Maintaining the optimal nucleotide balance required for normal cell proliferation is controlled by 5′-nucleotidases amongst other processes. These enzymes catalyze the dephosphorylation of ribo- and deoxyribonucleoside monophosphates to their corresponding nucleosides, and also exhibit, in certain cases phosphotransferase activity. All structures adopt a tetrameric assembly displaying a cross-like shape, in agreement with the quaternary solution structure. Each subunit consists of four domains: an “N-Terminal Regulatory Domain” (NTRD, M1 to K59), an “OD” (D60 to T143), a HAD-like Catalytic Domain (CD, F144 to K270 and K371 to Q444) and a C2 cap domain13 (K271 to N370).

The PfISN1-ΔC10 mutant truncated by ten residues at the C-terminus showed eightfold higher catalytic efficiency (kcat(app)/Km(app)) at pH 8 when lacking ATP and no change at pH 5.0. In the presence of ATP at pH 8, the activity was highly reduced. The structure of PfISN1-ΔC10 displays a PfISN1-ATP-bound like conformation (RMSD = 0.36 Å) confirming the role of LoopL430-Q444 as activity regulator. The ATP inhibiting effect on this variant suggests that the lack of LoopL430-Q444 allows binding of four ATPs at a time instead of two, resulting in a non-physiological intermediate. Upon mutation of H150 to V, PfISN1H150V-ΔC10 is no longer inhibited by ATP and PfISN1H150V-Apo is not activated by ATP. These observations confirm the role of H150 in ATP binding. Indeed in PfISN1H150V-Apo and PfISN1H150V-ΔC10, V150 can no longer interact with E419 and Y129, resulting in a reorganization of the effector site and an increase of the activity at pH 8.0 and 5.0.

>[2x]MKNLDINTFDNIEDIPLGSSEQDPYDFFTLSDRNVMNSDMKKNIVQWNSRYSYNQLKNKDSLIMFLVEIFRSLFVSNCIDKNIDNVLLSIEEMFIDHYYNPQHSRLKYLIDDVGIFFTKLPITKAFHTYNKKYRITKRLYAPPTFNEVRHILNLAQILSLEEGLDLLTFDADETLYPDGHDFNDEVLASYISCLLKKMNIAIVTAASYNNDAEKYQKRLENLLKYFSKHNIKDGSYKNFYVMGGESNYLFKCNEEATLYSVPENEWRHYKKFVDYDTVQEILNISEKCLEKVIKDFGLCAQIQRKEKSIGLVPNKIPSLNIKNEQKNYMIKYEVLEEAVIRIKKEIIKNKITAPYCAFNGGQDLWVDVGNKAEGLLILQKLLKIQKKKCCHIGDQFLHSGNDFPTRFCSLTLWVSNPQETKACLKSIMHLN>MTSVTSKQSTILGSDEIDLGRVIGELIDHRKLIISITSVFTLFAILYALLATPIYETDALIQIEQKQGNAILSSLSQVLPDGQPQSAPETALLQSRMILGKTIDDLNLQIQIEQKYFPVIGRGLARLMGEKPGNIDITRLYLPDSDDISNNTPSIILTVKDKENYSINSDGIQLNGVVGTLLNEKGISLLVNEIDAKPGDQFVITQLPRLKAISDLLKSFSVADLGKDTGMLTLTLTGDNPKRISHILDSISQNYLAQNIARQAAQDAKSLEFLNQQLPKVRAELDSAEDKLNAYRKQKDSVDLNMEAKSVLDQIVNVDNQLNELTFREAEVSQLYTKEHPTYKALMEKRQTLQEEKSKLNKRVSSMPSTQQEVLRLSRDVESGRAVYLQLLNRQQELNIAKSSAIGNVRIIDNAVTDPNPVRPKKTIIIVIGVVLGLIVSVVLVLFQVFLRRGIESPEQLEEIGINVYASIPISEWLTKNARQSGKVRKNQSDTLLAVGNPADLAVEAIRGLRTSLHFAMMEAKNNVLMISGASPSAGMTFISSNLAATIAITGKKVLFIDADLRKGYAHKMFGHKNDKGLSEFLSGQAAAEMIIDKVEGGGFDYIGRGQIPPNPAELLMHPRFEQLLNWASQNYDLIIIDTPPILAVTDAAIIGRYAGTCLLVARFEKNTVKEIDVSMKRFEQSGVVVKGCILNGVVKKASSYYRYGHNHYGYSEEDKKHHHHHH[8x]

Wzc, an integral cytoplasmic membrane tyrosine autokinase protein serves as the master regulator of the biosynthesis and export of many bacterial capsular polysaccharides and exopolysaccharides. Wzc comprises a large periplasmic domain, two transmembrane helices and a C-terminal cytoplasmic kinase domain with a tyrosine-rich tail. Wzc regulates polymerisation functions through cycling the formation and dissociation of an octameric complex, driven by changes in the phosphorylation status of the tyrosine-rich tail. E. coli Wzc serves a model for a wider family of polysaccharide co-polymerases.

Here, we report the characterisation of the structures WzcK540M2YE (Y718E, Y717E), WzcK540M3YE (Y718E, Y717E and Y715E) and WzcK540M3YE_N711Y (an additional N711Y mutation) corresponding to different phosphorylation states. When Y715 occupies the active site (1pY), Y713 is bound in the same pocket. The structural and MD data reported here confirm this hypothesis, showing that the tyrosine most stably positioned at the active site is the one immediately N-terminal to the phosphotyrosine (or the engineered Tyr-to-Glu mutation). We show that it is binding of the i-2 tyrosine to the tyrosine pocket (where i is the number of the residue positioned at the kinase active site) orders the tail between the tyrosine at the active site and helix α23. The presence of the negatively charged E675 in the tyrosine pocket we suggest is incompatible with binding a negatively charged phosphorylated tyrosine (or glutamic acid side chain). During the progressive phosphorylation sequence, the kinase domain is a rigid body. Structural alignment of the kinase domains of monomers of the full-length protein reveals increasing tilting of the transmembrane and periplasmic regions. When the octamer is viewed from the periplasm to the cytoplasm, progressive phosphorylation results in a clockwise rotation of transmembrane and periplasmic regions relative to the kinase ring. The movement of helix α1 is directly transmitted to transmembrane helix α2 and then to the periplasmic domain and, in this way, the phosphorylation signal from the cytoplasm is coupled to the periplasm.>[2x]MYAALFPGQGSHRVGMGRALYEASPAAKEVLDRAEAALPGLLKLMWEGPEEALTLTENQQPALLAAGYAAYRAFLEAGGKPPALAAGHSLGEWTAHVAAGTLELEDALRLVRLRGRYMQEAVPVGEGAMAAVLKLPLEEIQKALEGLEGVEIANLNAPEQTVISGRRQAVEEAAERLKERRARVVFLPVSAPFHSSLMAPARKRL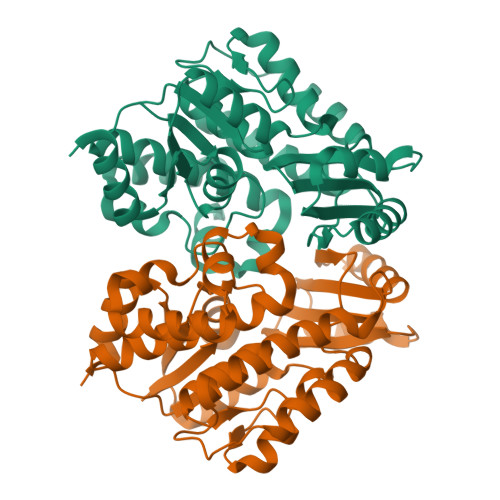AEDLAQVPLRRPRFPVYSNVTARPEEDPERIRALLLEQITAPVRWVEILRDMEARGVKRFLEFGSGEVLKGLVLRTLKEAEALSVQDPDSLRKALEVERA>MASLTVKAYLLGKEDAAREIRRFSFCCSPEPEAEAEAAAGPGPCERLLSRVAALFPALRPGGFQAHYRDEDGDLVAFSSDEELTMAMSYVKDDIFRIYIKEKKECRRDHRPPCAQEAPRNMV[3x]

PB1 domains are protein interaction modules with critical roles in the assembly of protein complexes involved in autophagy, signaling, cell division, and redox processes, as well as the auxin-response pathway in plants. PB1 domains form homotypic interactions via conserved electrostatic motifs molded by basic or acidic surface patches on opposite faces of their ubiquitin-like β-grasp fold. While type A and type B PB1 domains can form heterodimeric protein complexes, type AB members can mediate interactions with either PB1 domain type or engage in homotypic interactions to form homo-oligomers or hetero-oligomers. Our cryo-EM structures of filamentous p62 and AtNBR1–PB1 assemblies revealed that the presence of a tandem arginine sequence in the basic motif of type AB interfaces is required to stabilize a polymeric assembly.

Of the three PB1 assemblies studied, AtNBR11–94 (AtNBR1–PB1) and p621–122 (p62-PB1) formed homogeneous filaments of constant diameter that appeared best suited for high-resolution structure investigation by cryo-EM. Image classification of segmented PB1 helices revealed that both AtNBR1–PB1 and p62-PB1 polymerize in two different tubular morphologies: a projection class with a ladder-like pattern, we term L-type, and a projection class with a serpent-like one, we term S-type. Further analysis revealed that the occurrence of L-type or S-type assemblies is persistent along the individual helices in micrographs of AtNBR1–PB1, whereas for p62-PB1 filaments regularly displayed transitions from L-type to S-type symmetry. For p62-PB1, we observed a four-stranded L-type assembly and a three-stranded S-type assembly. In the latter S-type, one of the three helical rungs is propagating in an antiparallel orientation, related to the central rung by local dihedral symmetry. The L-type here has a pitch of 135.9 Å with 14.16 subunits/turn, and S-type has a pitch of 138.6 Å with 13.60 subunits/turn. Using the derived symmetries, we determined the 3.5/3.9- (L-type, p62/AtNBR1) and 4.0/4.4 Å- (S-type, p62/AtNBR1) resolution structures. All four structures form tubules of ~120 Å and 150-Å width with an inner diameter of 45 Å and 70 Å for AtNBR1–PB1 and p62-PB1, respectively. The main interactions are formed between a double arginine finger formed by two neighboring arginine residues in strand β2 (R19–R20AtNBR1/R21–22p62) stabilizing strong salt bridges to acidic residues (D60/D62/D64/D73AtNBR1 or D69/D71/D73/E82p62) in the OPCA motif located in the β2–β3 loop and the α2 helix. In addition to the canonical transverse interactions, the helices are further stabilized by longitudinal interactions Y14AtNBR1/N28AtNBR1 or K102p62/D92p62 and R59p62/D93p62 to subunits of neighboring strands along the helical axis.> MVYSYTEKKRIRKDFGKRPQVLDVPYLLSIQLDSFQKFIEQDPEGQYGLEAAFRSVFPIQSYSGNSELQYVSYRLGEPVFDVQECQIRGVTYSAPLRVKLRLVIYEREAPEGTVKDIKEQEVYMGEIPLMTDNGTFVINGTERVIVSQLHRSPGVFFDSDKGKTHSSGKVLYNARIIPYRGSWLDFEFDPKDNLFVRIDRRRKLPATIILRALNYTTEQILDLFFEKVIFEIRDNKLQMELVPERLRGETASFDIEANGKVYVEKGRRITARHIRQLEKDDVKLIEVPVEYIAGKVVAKDYIDESTGELICAANMELSLDLLAKLSQSGHKRIETLFTNDLDHGPYISETLRVDPTNDRLSALVEIYRMMRPGEPPTREAAESLFENLFFSEDRYDLSAVGRMKFNRSLLREEIEGSGILSKDDIIDVMKKLIDIRNGKGEVDDIDHLGNRRIRSVGEMAENQFRVGLVRVERAVKERLSLGDLDTLMPQDMINAKPI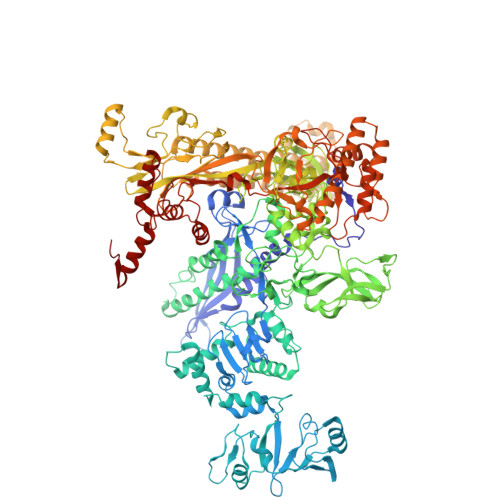SAAVKEFFGSSQLSQFMVQNNPLSEITHKRRISALGPGGLTRERAGFEVRDVHPTHYGRVCPIETPEGPNIGLINSLSVYAQTNEYGFLETPYRKVTDGVVTDEIHYLSAIEEGNYVIAQANSNLDEEGHFVEDLVTCRSKGESSLFSRDQVDYMDVSTQQVVSVGASLIPFLEHDDANRALMGANMQRQAVPTLRADKPLVGTGMERAVAVDSGVTAVAKRGGVVQYVDASRIVIKVNEDEMYPGEAGIDIYNLTKYTRSNQNTCINQMPCVSLGEPVERGDVLADGPSTDLGELALGQNMRVAFMPWNGYNFEDSILVSERVVQEDRFTTIHIQELACVSRDTKLGPEEITADIPNVGEAALSKLDESGIVYIGAEVTGGDILVGKVTPKGETQLTPEEKLLRAIFGEKASDVKDSSLRVPNGVSGTVIDVQVFTRDGVEKDKRALEIEEMQLKQAKKDLSEELQILEAGLFSRIRAVLVAGGVEAEKLDKLPRDRWLELGLTDEEKQNQLEQLAEQYDELKHEFEKKLEAKRRKITQGDDLAPGVLKIVKVYLAVKRRIQPGDKMAGRHGNKGVISKINPIEDMPYDENGTPVDIVLNPLGVPSRMNIGQILETHLGMAAKGIGDKINAMLKQQQEVAKLREFIQRAYDLGADVRQKVDLSTFSDEEVMRLAENLRKGMPIATPVFDGAKEAEIKELLKLGDLPTSGQIRLYDGRTGEQFERPVTVGYMYMLKLNHLVDDKMHARSTGSYSLVTQQPLGGKAQFGGQRFGEMEVWALEAYGAAYTLQEMLTVKSDDVNGRTKMYKNIVDGNHQMEPGMPESFNVLLKEIRSLGINIELEDE>MSCINLPTVLPGSPSKTRGQIQVILGPMFSGKSTELMRRVRRFQIAQYKCLVIKYAKDTRYSSSFCTHDRNTMEALPACLLRDVAQEALGVAVIGIDEGQFFPDIVEFCEAMANAGKTVIVAALDGTFQRKPFGAI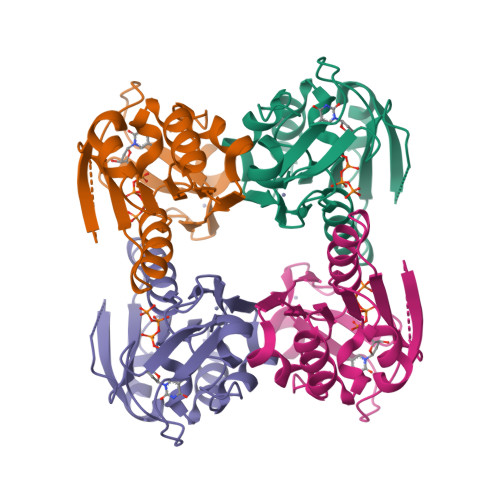LNLVPLAESVVKLTAVCMECFREAAYTKRLGTEKEVEVIGGADKYHSVCRLCYFKKASGQPAGPDNAANCPVPGKPGEAVAARKLFAPQQILQCSPAN[2x]>[2x]DKLIFAVDIIRHGDRTPIVALPTVNYQWQEGLGQLTAEGMQQ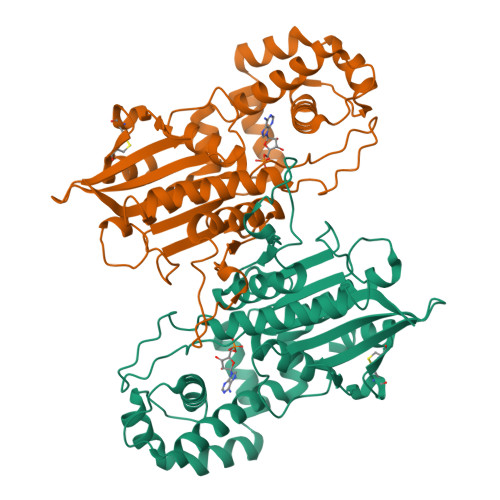EYKMGVAFRKKYIEESHLLPEHYEYGTIYVRSTDYARTLMSAQSLLMGLYPPGTGPTIPAGTSALPHAFQPIPVFSAPSKYDEVIIQQVDRKEREKLMEQYVFSTREWQQKNNELKDKYPLWSRLTGINIDNLGDLETVGHTLYIHQIHNAPMPEGLASNDIETIINSAEWAFMAQEKPQQIANVYSSKLMTNIADYLNSGSMKKSKLKYVLLSAHATTIASVLSFLGAPLEKSPPYASNVNFSLYDNGANYYTVKITYNGNPVSIPACGGSVCELQQLINLVHDS>[4x]MGSHHHHHHGRSMSELI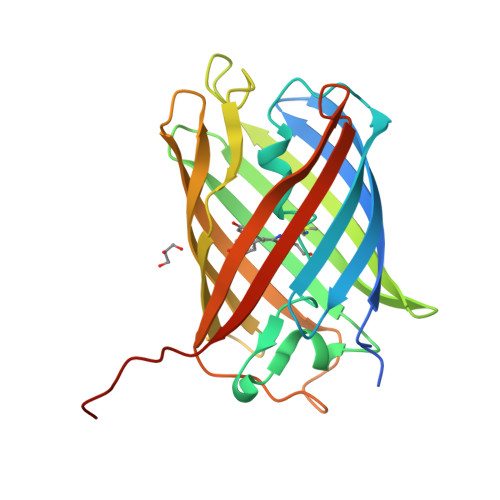KENMHMKLYMEGTVNNHHFKCTSEGEGKPYEGTQTMRIKVVEGGPLPFAFDILATSFMYGSYTFINHTQGIPDFFKQSFPEGFTWERVTTYEDGGVLTATQDTSLQDGCLIYNVKIRGVNFTSNGPVMQKKTLGWEAGTEMLYPADGGLEGRSDDALKLVGGGHLICNLKSTYRSKKPAKNLKVPGVYYVDRRLERIKEADKETYVEQHEVAVARYCDLPSKLGHKLN> KQFTKCELSQNLYDIDGYGRIALPELICTMFHTSGYDTQAIVENDESTEYGLFQISNALWCKSSQSPQSRNICDITCDKFLDDD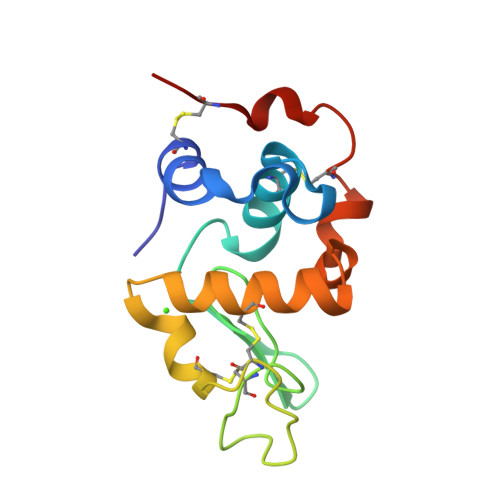ITDDIMCAKKILDIKGIDYWIAHKALCTEKLEQWLCEKE>APADNAADARPVDVSVSIFINKIYGVNTLEQTYKVDGYIVAQWTGKPRKTPGDKPLIVENTQIERWINNGLWVPALEFINVVGSPDTGNKRLMLFPDGRVIYNARFLGSFSNDMDFRLFPFDRQQFVLELEPFSYNNQQLRFSDIQVYTENIDNEEIDEWWIRGKASTHISDIRYDHLSSVQPNQNEFSRITVRIDAVRNPSYYLWSFILPLGLII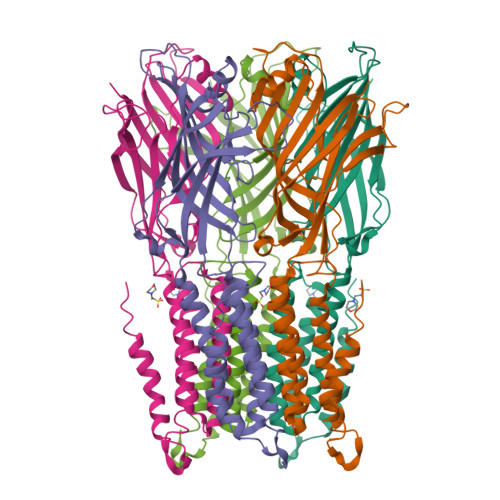AASWSVFWLESFSERLQTSFTLMLTVVAYAFYTSNILPRLPYTTVIDQMIIAGYGSIFAAILLIIFAHHRQANGVEDDLLIQRCRLAFPLGFLAIGCVLVIRGITL[10x]>MSLTLYQKKSKMIGIIIPDLNNRFYAQIIDGIQEVIQKEGYTALISFSTNSDVKKYQNAIINFENNNVDGIITSAFTIPPNFHLNTPLVMYDSANINDDIVRIVSNNT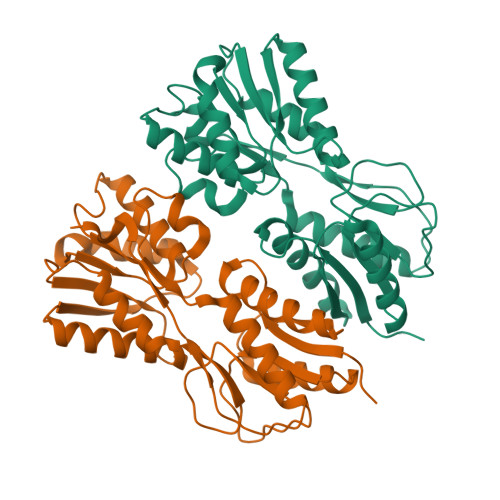KGGKESIKLLSKKIEKVLIQHWPLSLPTIRERIEAMTAEASKLKIDYLLEETPENNPYISAQSALNKSNQFDAIITVNDLYAAEIIKEAKRRNLKIPDDFQLVGYDNNILCGYTSPTISTIDQNPKLIGQTAAHRLLDLMSGNNSTRNSIIDVLPIKRDSTEGHHHHHH[2x]>[2x]SHMNSPLAPVGVFDSGVGGLTVARAI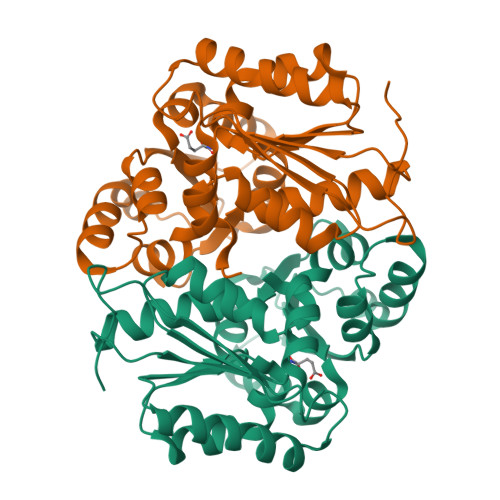IDQLPDEDIVYVGDTGNGPYGPLTIPEIRAHALAIGDDLVGRGVKALVIACNSASSACLRDARERYQVPVVEVILPAVRRAVAATRNGRIGVIGTRATITSHAYQDAFAAARDTEITAVACPRFVDFVERGVTSGRQVLGLAQGYLEPLQRAEVDTLVLGCTHYPLLSGLIQLAMGENVTLVSSAEETAKEVVRVLTEIDLLRPHDAPPATRIFEATGDPEAFTKLAARFLGPVLGGVQPVHPSRIH>MQIPASEQETLVRPKPLLLKLLKSVGAQKDTYTMKEVLFYLGQYIMTKRLYDEKQQHIVYCSNDL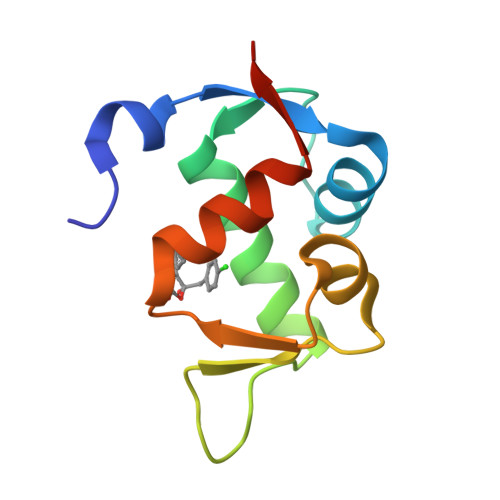LGDLFGVPSFSVKEHRKIYTMIYRNLVVVNQQE[2x]> QSTRVEEGSKVAISCSLMADEGVHWFRQGKKPNPEFLVYISGIGSQNPAAKDKYSADKSSQKVTLTVKDFRKEDSGKYYCLMVKNRALTFGKPQDYY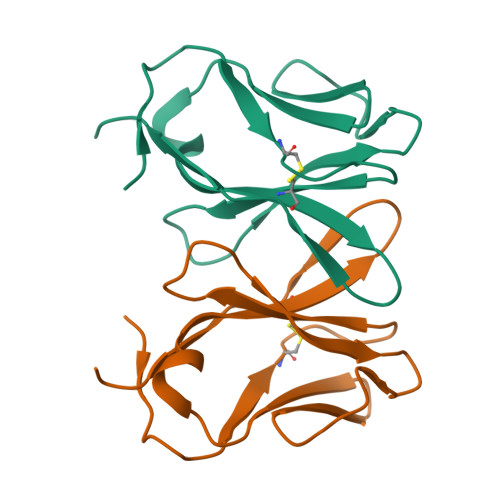VEE> GRTCPKPDD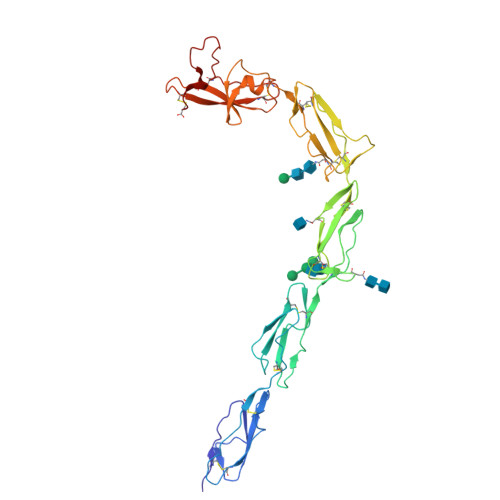LPFSTVVPLKTFYEPGEEITYSCKPGYVSRGGMRKFICPLTGLWPINTLKCTPRVCPFAGILENGAVRYTTFEYPNTISFSCNTGFYLNGADSAKCTEEGKWSPELPVCAPIICPPPSIPTFATLRVYKPSAGNNSLYRDTAVFECLPQHAMFGNDTITCTTHGNWTKLPECREVKCPFPSRPDNGFVNYPAKPTLYYKDKATFGCHDGYSLDGPEEIECTKLGNWSAMPSCKASCKLPVKKATVVYQGERVKIQEKFKNGMLHGDKVSFFCKNKEKKCSYTEDAQCIDGTIEVPKCFKEHSSLAFWKTDASDVKPC>GSMDYKRRIHKFQAHFGKKGFEGALVAPGSNFYYLTGFNPLGTLERLFVLILPSEGLLTAIAPRLYEKELEEFNGEVVLWSDSENPYKIFATKIKETFKEGEKLLIDDTMPVGVFLKAKDIFDKYSLHPISPVISELREIKDKDEIKAHKKAAEIVDKVFYRFIEGKLEGKSERELANRIEYMIKNEFGADDVSFEPIVASGPNGANPHHRPSHRKIRKGDVVIFDYGAKYLGYCSDVTRTVVVGPPSEEVKKVYEIVKEAQETAVQKVAEGIPAEVVDATARGIISKYGYGEYFIHRTGHGLGIDVHEEPYISPGNK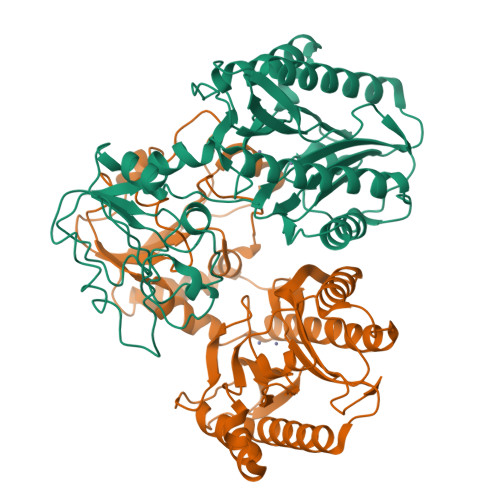KILKDGMVFTIEPGIYLQGKFGVRIEDDVALVDKKGIRLTNADRELITL[4x]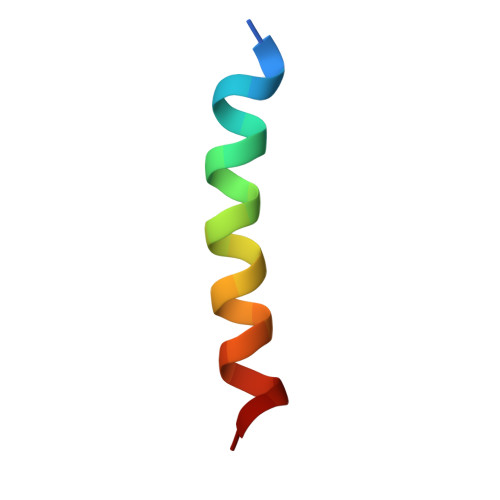> EVIPMAAVKQALREAGDEFELRYR> MAWSHPQFEKIEGRMEEGARHRNNTEKKHPGGGESDASPEAGSGGGGVALKKEIGLVSACGIIVGNIIGSGIFVSPKGVLENAGSVGLALIVWIVTGFITVVGALCYAELGVTIPKSGGDYSYVKDIFGGLAGFLRLWIAVLVIYPTNQAVIALTFSNYVLQPLFPTCFPPESGLRLLAAICLLLLTWVNCSSVRWATRVQDIFTAGKLLALALIIIMGIVQICKGEYFWLEPKNAFENFQEPDIGLVALAFLQGSFAYGGWNFLNYVTEELVDPYKNLPRAIFISIPLVTFVYVFANVAYVTAMSPQELLASNAVAVTFGEKLLGVMAWIMPISVALSTFGGVNGSLFTSSRLFFAGAREGHLPSVLAMIHVKRCTPIPALLFTCISTLLMLVTSDMYTLINYVGFINYLFYGVTVAGQIVLRWKKPDIPRPIKINLLFPIIYLLFWAFLLVFSLWSEPVVCGIGLAIMLTGVPVYFLGVYWQHKPKCFSDFIELLTLVSQKM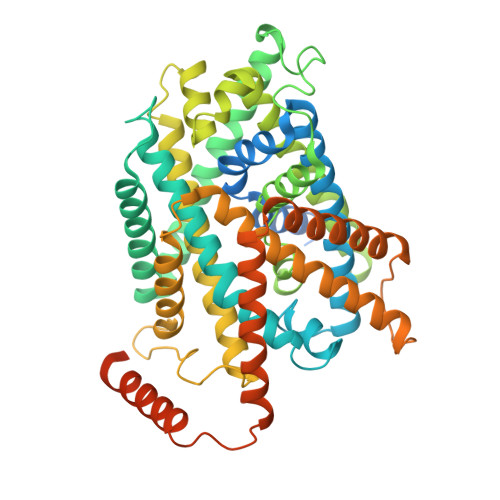CVVVYPEVERGSGTEEANEDMEEQQQPMYQPTPTKDKDVAGQPQP Clustered protocadherins (cPcdhs) are a large family of cadherin-like proteins named for the clustered arrangement of their genes in vertebrate genomes. cPcdhs play roles in many facets of neural development, including circuit development, most notably neurite self-avoidance in vertebrates, and tiling. In mammalian nervous systems, cPcdh isoform expression is controlled by the unique organization of three tandem gene clusters, Pcdhα, Pcdhβ, and Pcdhγ, with each cluster containing multiple variable exons, which encode full cPcdh ectodomain regions with six extracellular cadherin (EC) domains, a single transmembrane region, and a short cytoplasmic extension. The last two variable exons in the Pcdhα gene cluster and the last three variable exons of the Pcdhγ gene cluster diverge in sequence from other cPcdh isoforms and are referred to as ‘C-type’ cPcdhs. Moreover, Garrett et al. discovered that neuronal survival and postnatal viability are controlled solely by γC4 suggesting a function that is unique to this isoform (although it presumably requires β and/or other γ carriers to reach the cell surface).

The biophysical properties of C-type cPcdhs pose a number of interesting questions: Despite their more divergent sequences compared with alternate cPcdhs, AUC data have confirmed that C-type cPcdhs αC2, γC3, and γC5 form trans dimers using their EC1–4 domains. However, γC41–4 behaved as a very weak dimer in AUC (KD >500 μM; Figure 2—source data 1), nevertheless full-length γC4 can mediate cell aggregation when delivered to the cell surface by coexpression with a ‘carrier’ cPcdh. However, there are no published crystal structures of C-type cPcdh trans dimers. We therefore sought to crystallize a mouse C-type cPcdh engaged in a trans interaction and obtained two distinct crystal forms of γC4EC1–4, one at 2.4 Å resolution (crystallized at pH 7.5) and the other with anisotropic diffraction at 4.6/3.9/3.5 Å resolution (Figure 3—source data 1) (crystallized at pH 6.0). However, the 2.4 Å structure had an apparently partially disrupted EC2:EC3 interface resulting in a total buried surface area of just 2900 Å2. Left, surface views of the two trans dimer crystal structures highlight the difference, with a gap apparent in the EC2:EC3 region of the interface in crystal form two that is absent from crystal form 1. The difference between the two structures may be due to differences in the pH of the crystallization and its effect on the ionization state of the three histidines present in the EC2:EC3 interface. The differences could also reflect distinct states of a dynamic interaction, as has previously been observed crystallographically and explored computationally for other cPcdh trans interactions. The published crystal structures of γA1, γA8, and γB3 also show partially disrupted trans interfaces though in differing regions of the interface (Goodman et al., 2016a, Nicoludis et al., 2016).

>QIRYPVPEESQEGTFVGNVAQDFLLDTESLSARRLQVAGEVNQRHFRVDLDSGALLIKNPIDREALCGLSASCIVPLEFVTEGPLEMYRAEVEIVDVNDHAPRFPRQQLDLEIGEAAPPGQRFPLEKAQDADVGSNSISSYRLSSNEHFALDVKKRSDGSLVPELLLEKPLDREKQSDYRLVLTAVDGGNPPRSGTAELRVSVLDVNDNAPAFQQSSYRISVLESAPAGMVLIQLNASDPDLGPSGNVTFSFSGHTPDRVRNLFSLHPTTGKLTLQGPLDFESENYYEFDVRARDGGSPAMEQHCSLRVDLLDVNDNAPHITVTSELGTLPESAEPGTVVALISVQDPDSGSNGDVSLRIPDHLPFALKSAFRNQFSLVTAGPLDREARSSYDIMVTASDAGNPPLSTHRTIFLNISDVNDHHHHHHHH[2x]>AESLPDLKIEKLDEGVYVHTSFEEVNGWGVVPKHGLVVLVNAEAYLIDTPFTAKDTEKLVTWFVERGYKIKGSISSHFHSDSTGGIEWLNSRSIPTYASELTNELLKKDGKVQATNSFSGVNYWLVKNKIEV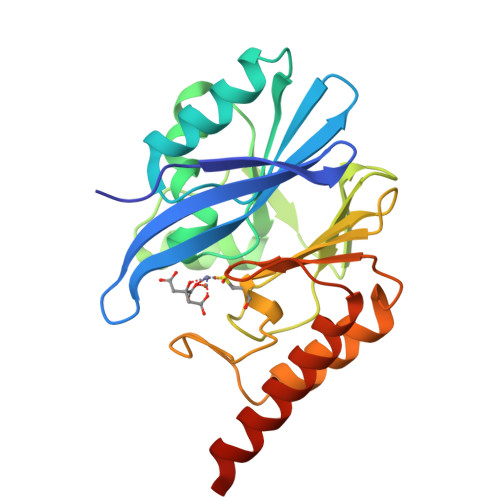FYPGPGHTPDNVVVWLPERKILFGGCFIKPYGLGNLGDANIEAWPKSAKLLKSKYGKAKLVVPSHSEVGDASLLKLTLEQAVKGLNESKKPSKPSN[4x]>[4x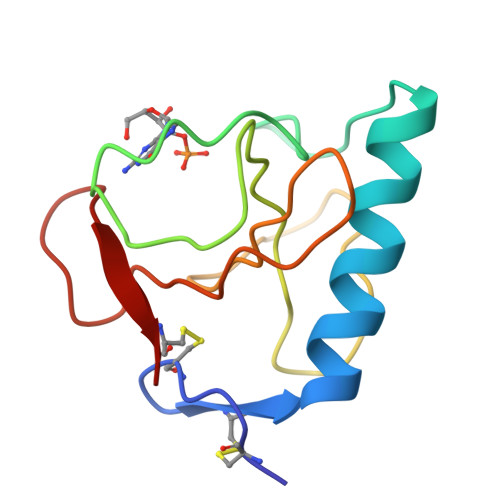]ACDYTCGSNCYSSSDVSTAQAAGYKLHEDGETVGSNSYPHKYNNYEGFDFSVSSPYYEWPILSSGDVYSGGSPGADRVVFNENNQLAGVITHQGASGNNFVECT> MKKIILTIGCPGSGKSTWAREFIAKNPGFYNINRDDYR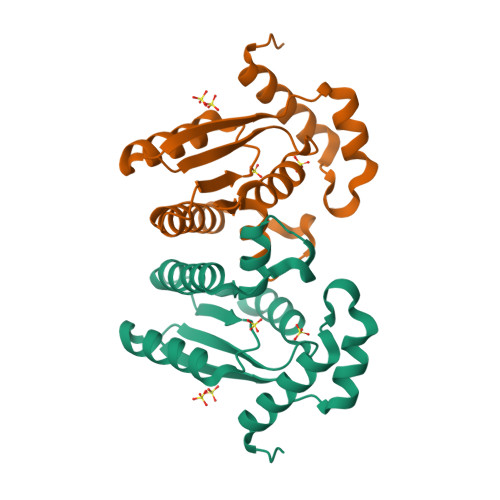QSIMAHEERDEYKYTKKKEGIVTGMQFDTAKSILYGGDSVKGVIISDTNLNPERRLAWETFAKEYGWKVEHKVFDVPWTELVKRNSKRGTKAVPIDVLRSMYKSMREYLGLPVYNGTPGKPKAVIFDVDGTLAKMNGRGPYDL AsfvPCNA is a hypothetic sliding clamp family protein; it is coded by the E301R gene that is highly conserved in ASFV strains. The crystal structures were determined at atomic resolution and confirmed that AsfvPCNA can assemble into a homotrimeric ring-shaped structure. Different from homologous protein structures, AsfvPCNA has a very unique amino acid sequence and conformation at the IDCL, J-loop, and P-loop regions, which are involved in partner recognition by PCNAs. Although the detailed molecular basis remains to be investigated, AsfvPCNA has a high dsDNA-binding affinity and can enhance the catalytic activity of the AsfvLIG protein, which plays critical roles in both DNA replication and DNA repair pathways of ASFV.

Using the purified AsfvPCNA protein, we performed extensive crystallization trials and solved the structures in two different forms, Form I and Form II. Unlike the Form I structure, the Form II AsfvPCNA structure belongs to P1 space group; per asymmetric unit contains six AsfvPCNA molecules, which assemble into two homotrimeric ring structures. The overall conformations of Form I and Form II AsfvPCNA trimers are virtually identical, supported by the very low root mean square deviation (RMSD, 0.2 Å) value over 840 pairs of Cα atoms. The three AsfvPCNA protomers arrange in a head-to-tail fashion, embracing all Domain I and Domain II α-helices at the inner face of the ring. The diameter of the inner ring is approximately 30 Å. We could not obtain any AsfvPCNA crystal in the absence of dsDNA, whereas Form I and Form II AsfvPCNA crystals readily grew when 10 bp dsDNA (5′-CCCATCGTAT-3′; 5′-ATACGATGGG-3′) is present in the sample. In the structures, extra electron density maps could be observed in the central channel, suggesting the existence of dsDNA. Likely, due to the dynamic binding or sliding of the DNA, the electron density is diffused, and no DNA was included in the final structures. Although it is ordered in the 7DRH structure, the four residues (298NNTI301) are all disordered in the Form I and Form II AsfvPCNA structures, suggesting that AsfvPCNA C-tail is very flexible and can undergo large conformational changes in solution.

>GSMSEDIRRGPGRPPKKRVVPNFERKGILEKPVRPQSRLEFSYDNPLIFKNLFIYFKNLKSKNILVRCTPTEITFFSRDQSQASFVIATIDGKNVNHYYASDVFWLGINRELVEKMFNSIDRSFLKITIVHRYDKPETLFFIFTDFDIDKECTYQITVSEPELDMDLIEMEKSISEERLKNYPLRWEFTSKQLKKTFSDLSNYTELVTIEKLGGDTPLHLYFQKFNSISYHEMYKSSNKINLTSTIPKSQVFQINVKIAHIKSLASAMVTDKIRILCEENGNLIFQSEMDALMLNTITLNNTI[6x]> MEHVAFGSEDIENTLAKMDDGQLDGLAFGAIQLDGDGNILQYNAAEGDITGRDPKQVIGKNXFKDVAPCTDSPEFYGKFKEGVASGNLNTMFE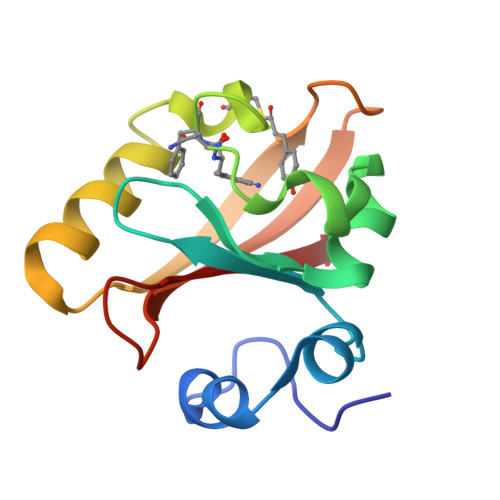YTFDYQMTPTKVKVHMKKALSGDSYWVFVKRV4-PHOSPHO-D-ERYTHRONATE | C4 H9 O8 P | 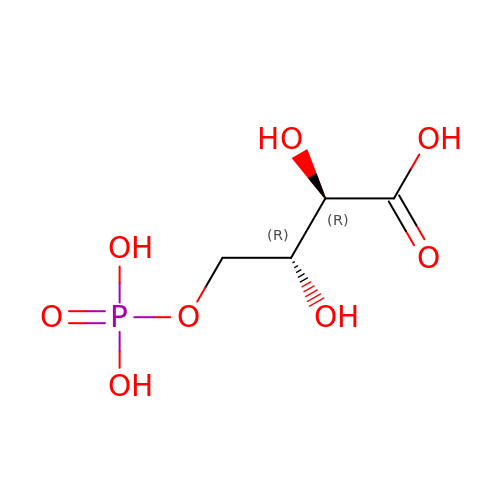ZCZXOHUILRHRQJ-PWNYCUMCSA-N>GSHMGRPSSKEGRRSDTCEYCGKVFKNCSNLTVHRRSHTGERPYKCELCNYACAQSSKLTRHMKTHGQVGKDVYKCEICKMPFSVYSTLEKHMKKWHSDRVL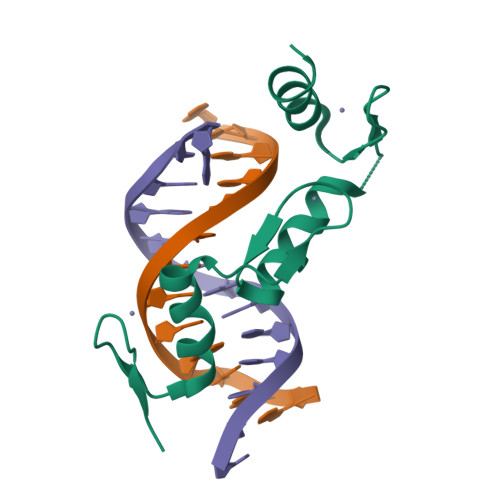NNDIKTE[2x]> SAKGIDYDKLIVRFGSSKIDKELINRIERATGQRPHHFLRRGIFFSHRDMNQVLDAYENKKPFYLYTGRGPSSEAMHVGHLIPFIFTKWLQDVFNVPLVIQMTDDEKYLWKDLTLDQAYSYAVENAKDIIACGFDINKTFIFSDLDYMGMSSGFYKNVVKIQKHVTFNQVKGIFGFTDSDCIGKISFPAIQAAPSFSNSFPQIFRDRTDIQCLIPCAIDQDPYFRMTRDVAPRIGYPKPALLHSTFFPALQGAQTKMSASDPNSSIFLTDTAKQIKTKVN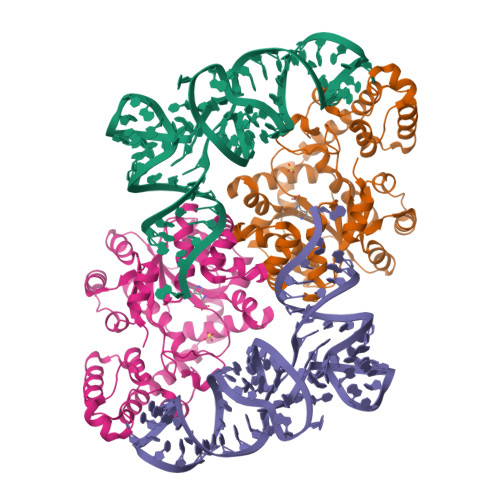KHAFSGGRDTIEEHRQFGGNCDVDVSFMYLTFFLEDDDKLEQIRKDYTSGAMLTGELKKALIEVLQPLIAEHQARRKEVTDEIVKEFMTPRKLSFDFQHHHHHH> PISPIETVPVKLKPGMDGPKVKQWPLTEEKIKALVEICTEMEKEGKISKIGPENPYNTPVFAIKKKDSTK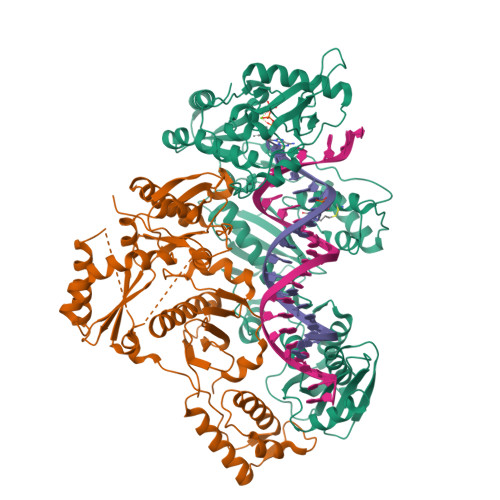WRKLVDFRELNKRTQDFWEVQLGIPHPAGLKKKKSVTVLDVGDAYFSVPLDEDFRKYTAFTIPSINNETPGIRYQYNVLPQGWKGSPAIFQSSMTKILEPFRKQNPDIVIYQYMDDLYVGSDLEIGQHRTKIEELRQHLLRWGLTTPDKKHQKEPPFLWMGYELHPDKWTVQPIVLPEKDSWTVNDICKLVGKLNWASQIYPGIKVRQLSKLLRGTKALTEVIPLTEEAELELAENREILKEPVHGVYYDPSKDLIAEIQKQGQGQWTYQIYQEPFKNLKTGKYARMRGAHTNDVKQLTEAVQKITTESIVIWGKTPKFKLPIQKETWETWWTEYWQATWIPEWEFVNTPPLVKLWYQLEKEPIVGAETFYVDGAANRETKLGKAGYVTNRGRQKVVTLTDTTNQKTELQAIYLALQDSGLEVNIVTDSQYALGIIQAQPDQSESELVNQIIEQLIKKEKVYLAWVPAHKGIGGNEQVDKLVSAGIRKVL;> PISPIETVPVKLKPGMDGPKVKQWPLTEEKIKALVEICTEMEKEGKISKIGPENPYNTPVFAIKKKDSTKWRKLVDFRELNKRTQDFWEVQLGIPHPAGLKKKKSVTVLDVGDAYFSVPLDEDFRKYTAFTIPSINNETPGIRYQYNVLPQGWKGSPAIFQSSMTKILEPFRKQNPDIVIYQYMDDLYVGSDLEIGQHRTKIEELRQHLLRWGLTTPDKKHQKEPPFLWMGYELHPDKWTVQPIVLPEKDSWTVNDIQKLVGKLNWASQIYPGIKVRQLSKLLRGTKALTEVIPLTEEAELELAENREILKEPVHGVYYDPSKDLIAEIQKQGQGQWTYQIYQEPFKNLKTGKYARMRGAHTNDVKQLTEAVQKITTESIVIWGKTPKFKLPIQKETWETWWTEYWQATWIPEWEFVNTPPLVKLWYQLEKEPIVGAETF4-propylbenzoic acid | C10 H12 O2 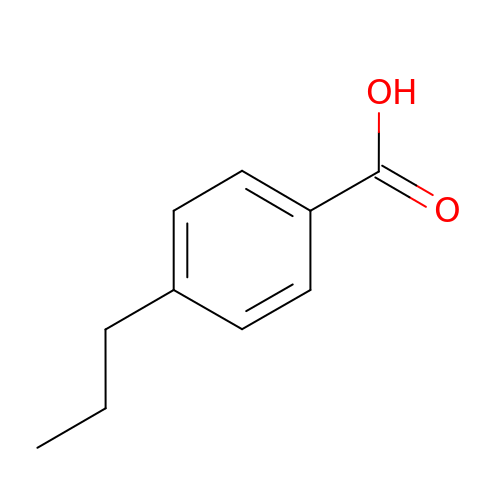| ATZHGRNFEFVDDJ-UHFFFAOYSA-N>[2x]MKMTSIQQRAELHRQIWQIANDVRGSVDGWDFKQYVLGALFYRFISENFSSYIEAGDDSICYAKLDDSVITDDIKDDAIKTKGYFIYPSQLFCNVAAKANTNDRLNADLNSIFVAIESSAYGYPSEADIKGLFADFDTTSNRLGNTVKDKNARLAAVLKGVEGLKLGDFNEHQIDLFGDAYEFLISNYAANAGKSGGEFFTPQHVSKLIAQLAMHGQTHVNKIYDPAAGSGSLLLQAKKQFDNHIIEEGFFGQEINHTTYNLARMNMFLHNINYDKFDIKLGNTLTEPHFRDEKPFDAIVSNPPYSVKWIGSDDPTLINDERFAPAGVLAPKSKADFAFVLHALNYLSAKGRAAIVCFPGIFYRGGAEQKIRQYLVDNNYVETVI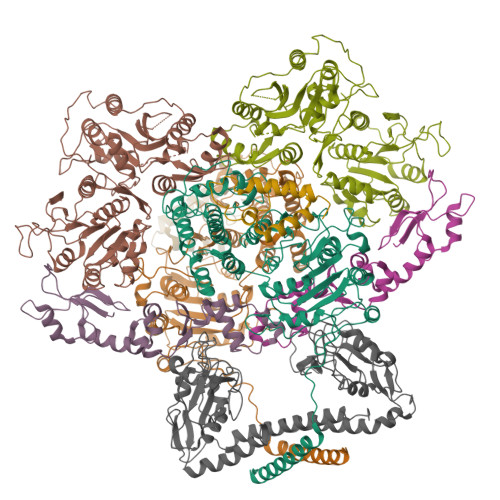SLAPNLFFGTTIAVNILVLSKHKTDTNVQFIDASELFKKETNNNILTDAHIEQIMQVFASKEDVAHLAKSVAFETVVANDYNLSVSSYVEAKDNREIIDIAELNAELKTTVSKIDQLRKDIDAIVAEIEGCEVQK;>[4x]MTHQTHTIAESNNFIVLDKYIKAEPTGDSYQSESDLERELIQDLRNQGYEFISVKSQSAMLANVREQLQNLNGVVFNDSEWRRFTEQYLDNPSDGILDKTRKIHIDYICDFIFDDERLENIYLIDKKNLMRNKVQIIQQFEQAGSHANRYDVTILVNGLPLVQIELKKRGVAIREAFNQIHRYSKESFNSENSLFKYLQLFVISNGTDTRYFANTTKRDKNSFDFTMNWAKSDNTLIKDLKDFTATCFQKHTLLNVLVNYSVFDSSQTLLVMRPYQIAATERILWKIKSSFTAKNWSKPESGGYIWHTTGSGKTLTSFKAARLATELDFIDKVFFVVDRKDLDYQTMKEYQRFSPDSVNGSENTAGLKRNLDKDDNKIIVTTIQKLNNLMKAESDLPVYNQQVVFIFDECHRSQFGEAQKNLKKKFKRYYQFGFTGTPIFPENALGSETTASVFGRELHSYVITDAIRDEKVLKFKVDYNDVRPQFKSLETETDEKKLSAAENQQAFLHPMRIQEITQYILNNFRQKTHRTFPGSKGFNAMLAVSSVDAAKAYYATFKRLQEEAANKSATYKPLRIATIFSFAANEEQNAIGEISDETFDTSAMDSSAKEFLDAAIREYNSHFKTNFSTDSNGFQNYYRDLAQRVKNQDIDLLIVVGMFLTGFDAPTLNTLFVDKNLRYHGLMQAFSRTNRIYDATKTFGNIVTFRDLERSTIDAITLFGDKNTKNVVLEKSYTEYMEGFTDAATGEAKRGFMTVVSELEQRFPDPTSIESEKEKKDFVKLFGEYLRAENILQNYDEFATLKALQQIDLSDPVAVEKFKAEHYVDDEKFAELQTIRLPADRKIQDYRSAYNDIRDWQRREKEAEKKEKSTTDWDDVVFEVDLLKSQEINLDYILGLIFEHNRQNKGKGEMIEEVKRLIRSSLGNRAKEGLVVDFIQQTNLDDLPDKASIIDAFFTFAQREQQREAEALIKEENLNEDAAKRYIRTSLKREYATENGTELNETLPKLSPLNPQYKTKKQAVFQKIVSFIEKFKGVGGKI;>[2x]MDDMQVYIANLGKYNEGELVGAWFTFPIDFEEVKEKIGLNDEYEEYAIHDYELPFTVDEYTSIGELNRLWEMVSELPEELQSELSALLTHFSSIEELSEHQEDIIIHSDCDDMYDVARYYIEETGALGEVPASLQNYIDYQAYGRDLDLSGTFISTNHGIFEIVY;> MSEMSYLEKLLDGVEVEWLPLGEITKYEQPTKYLVKAKDYHDTYTIPVLTAGKTFILGYTNETHGIYQASKAPVIIFDDFTTANKWVDFDFKAKSSAMKMVTSCDDNKTLLKYVYYWLNTLPSEFAEGDHKRQWISNYSQKKIPIPCPDNPEKSLAIQSEIVRILDKFTALTAELTAELNMRKKQYNYYRDQLLSFKEGEVEWKTLGEIGKWYGGGTPSKNKIEFWENGSIPWISPKDMGRTLVDSSEDYITEEAVLHSSTKLIPANSIAIVVRSSILDKVLPSALIKVPATLNQDMKAVIPHENILVKYIYHMIGSRGSDILRAAKKTGGSVASIDSKKLFSFKIPVPNINEQQRIVEILDKFDTLTNSITEGLPREIELRQKQYEYYRDLLFSFPKPETVSN(5-hydroxy-6-methylpyridin-3-yl)methyl dihydrogen 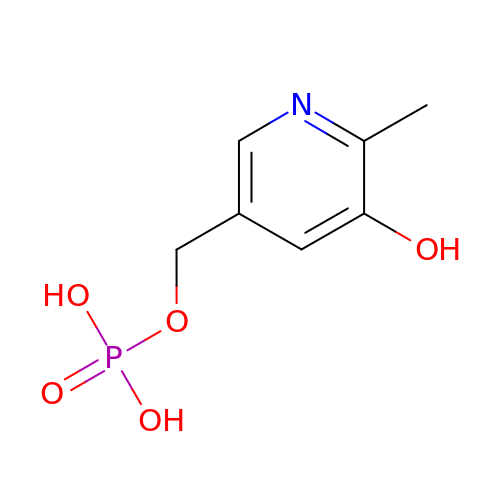phosphate | C7 H10 N O5 P | CKIPHKBHPIDPOG-UHFFFAOYSA-N> MKFLKNVLEEGSKLEEFNELELSPEDKELLEYLQQTKAKITVVGCGGAGNNTITRLKMEGIEGAKTVAINTDAQQLIRTKADKKILIGKKLTRGLGAGGNPKIGEEAAKESAEEIKAAIQDSDMVFITCGLGGGTGTGSAPVVAEISKKIGALTVAVVTLPFVMEGKVRMKNAMEGLERLKQHTDTLVVIPNEKLFEIVPNMPLKLAFKVADEVLINAVKGLVELITKDGLINVDFADVKAVMNNGGLAMIGIGESDSEKRAKEAVSMALNSPLLDVDIDGATGALIHVMGPEDLTLEEAREVVATVSSRLDPNATIIWGATIDENL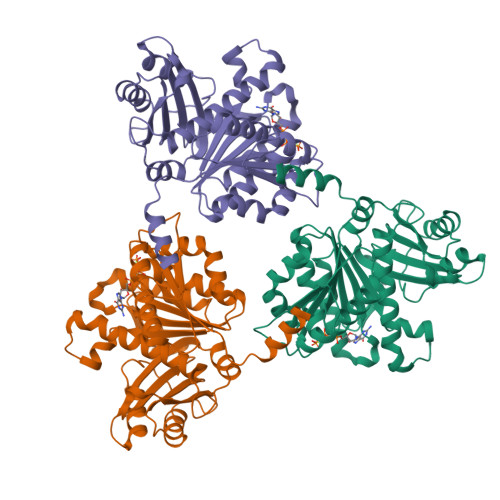ENTVRVLLVITGVQSRIEFTDTGLKRKKLELTGIPKI> MRRVSPLERIRLFGRAGLDVVAALGRSTLFLGHALLGRRTPGTGLHLLVKQLYSVGVLSLAIIVVSGLFIGMVLALQGYNILISYGSEQ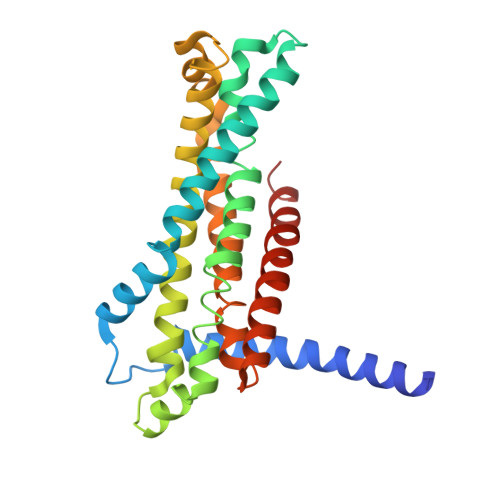AVGQMVALTLLRELGPVVTGLLFAGRAGSALTAEIGNMKATEQLSSLEMIGVDPLKYIVAPRLWAGFISMPLLAAIFSVVGIWGGAMVAVDWLGVYEGSFWANMQNSVQFTEDVLNGVIKSIVFAFVVTWIAVYQGYDCEPTSEGISRATTRTVVYASLAVLGLDFILTALMFGDF>MEMMIKKRIKQVKKGDQDAFADIVDIYKDKIYQLCYRMLGNVHEAEDIAQEAFIRAYVNIDSFDINRKFSTWLYRIATNLTIDRIRKKKPDYYLDAEVAGTEGLTMYSQIVADGVLPEDAVVSLELSNTIQQKILKLP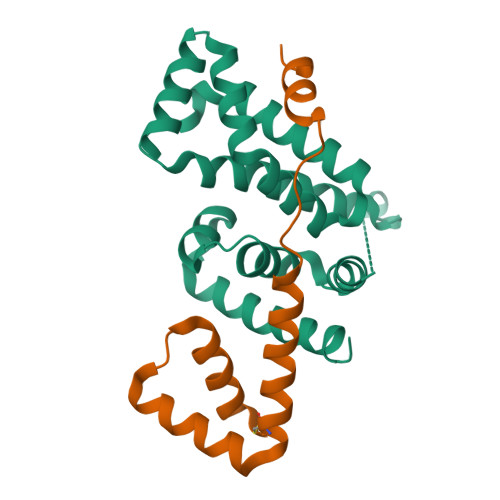DKYRTVIVLKYIDELSLIEIGEILNIPVGTVKTRIHRGREALRKQLRDL[2x];>[2x]MSCPEQIVQLMHMHLDGDILPKDEHVLNEHLETCEKCRKHFYEMEKSIALVRSTSHVEAPADFTANVMAKLPKEKKRASV>LPNITILATGGDIAGGGDSATKSNYTVGKVGVENLVNAVPQLKDIANVKGEQVVNIGSQDMNDNVWLTLAKKINTDCDKTDGFVITHGVDTMEETAYFLDLTVKCDKPVVMVGAMRPSTSMSADGPFNLYNAVVTAADKASANRGVLVVMNDTVLDGRDVTKTNTTDVATFKSVNYGPLGYIHNGKIDYQRTPARKHTSDTPFDVSKLNELPKVGIVYNYANASDLPAKALVDAGYDGIVSAGVGNGNLYKSVFDTLATAAK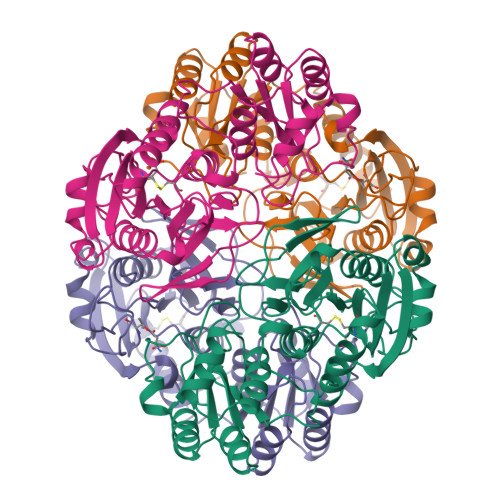TGTAVVRSSRVPTGATTQDAEVDDAKYGFVASGTLNPQKARVLLQLALTQTKDPQQIQQIFNQY[4x]> MGSSHHHHHHSSGENLYFQGSK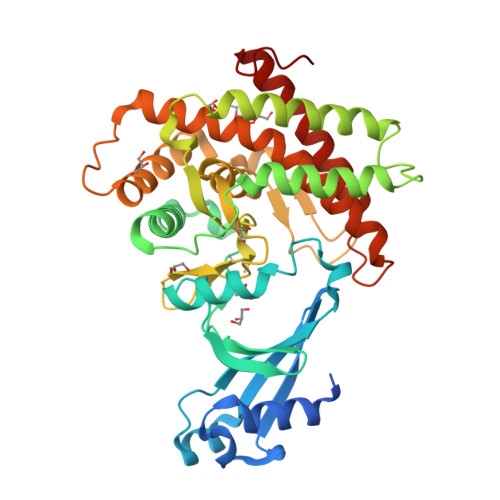LTDPLYIKKICLEKVHDWSRCNEDDVCVNQILSGLTNQLFEVSIKEDTAIEYRITRRHVLFRIYGKDVDALYNPLSEFEVYKTMSKYRIAPLLLNTFDGGRIEEWLYGDPLSIDDLKNKSILVGIANVLGKFHTLSRKRHLPEHWDKTPCVFKMMDRWRLAVSNYKNLDKVTLDINKYIQESHKFLKFIKIYTQIENIANDIVFCHNDLQENNIMNTNKCLRLIDFEYSGYNFLSADIANFFIETTIDYSYNAYPFFIINKKNYISYESRILFVTTYLSKYLDDSTAASDQDIIDQFLEAIEVQALGLHLIWAFWSIIRGYQTKSYNEFDFFLYAKERLKMYDEQKQYLMSKNIIKDYDD>MAGRTRIPFNGVGTSVLPAYQTLSAGQYLLSPNQRFKLLLQGDGNLVIQDNGATVWVANEQQPFSSTIPLRNKKAPLAFYVQYGAFLDDYSRRRVWLTDNSTFTSNDQWNRTHLVLQDDGNIVLVDSLALWNGTPAIPLVPGAIDSLLLAPGSELVQGVVYGAGASKLVFQGDGNLVAYG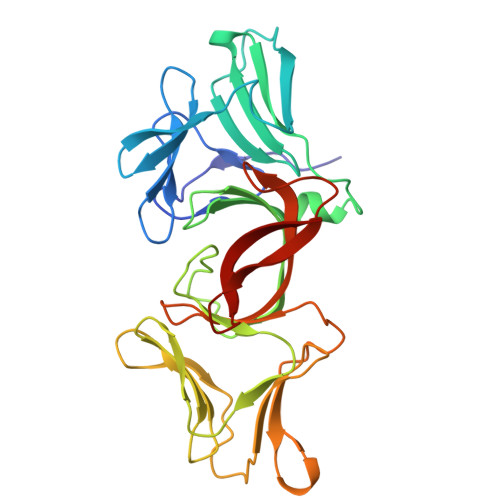PNGAATWNAGTQGKGAVRAVFQGDGNLVVYGAGNAVLWHSHTGGHASAVLRLQANGSIAILDEKPVWARFGFQPTYRHIRKINPDQKPIDIWTWHF[2x]> MQQQCDTVSAWQSLRGPGTGGYYLFKTTEGGKTDCTYVKGSNFNDAAQTATYTYGNMGSGNQMTQQTASASISGNAIVVGTDHSEVMYSDGSTCDVV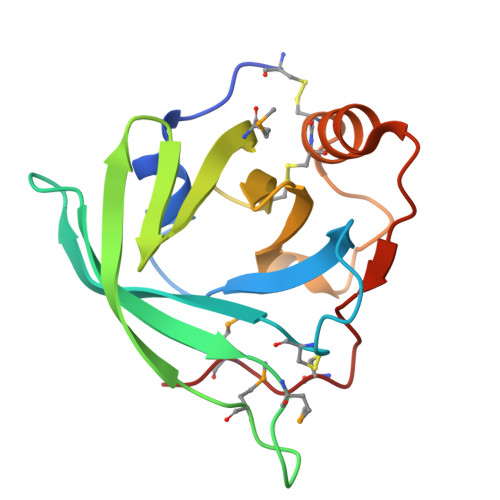RLNGQIELWIHSSATSNTGNLNSCCTDKFNQEKGSRPEHVVYRSTCPNMPQ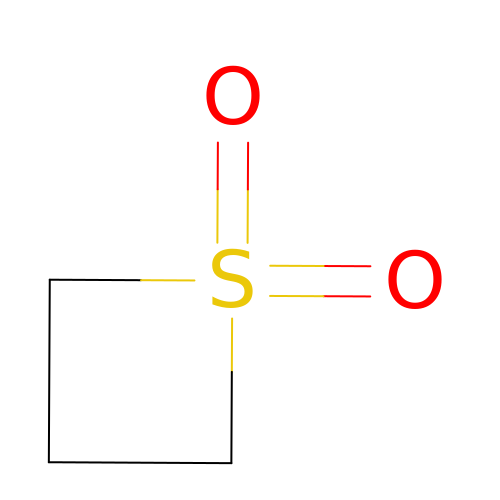1lambda~6~-thietane-1,1-dione | C3 H6 O2 S | FCFMKFHUNDYKEG-UHFFFAOYSA-N>[4x]MGSDKIHHHHHHENLYFQGMTIAEIAKDFTELLKQGDNAGAAEKYNADDIASYEAMEGPMAVSHGKEALRQKSQW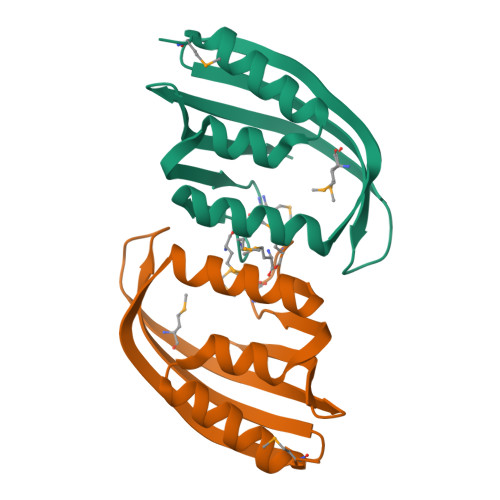WQENHEVHGGSVEGPYVNGDQFALRFKFDVTPKATGERVTMDEVGLYTVKNGKITEERFYY> DEKRLHFGNGHLKLPGLRTYVDPHTYEDPTQTVHEFAKELDATNISIDKVVGAGEFGEV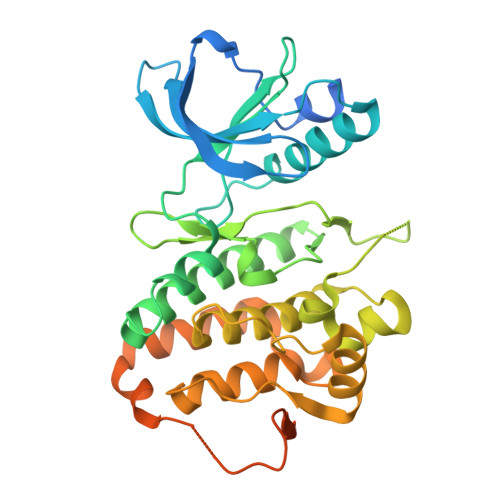CSGRLKLPSKKEISVAIKTLKVGYTEKQRRDFLGEASIMGQFDHPNIIRLEGVVTKSKPVMIVTEYMENGSLDSFLRKHDAQFTVIQLVGMLRGIASGMKYLSDMGYVHRDLAARNILINSNLVCKVSDFGLSRVLEDDPEAAYTTRGGKIPIRWTSPEAIAYRKFTSASDVWSYGIVLWEVMSYGERPYWEMSNQDVIKAVDEGYRLPPPMDCPAALYQLMLDCWQKDRNNRPKFEQIVSILDKLIRNPGSLKIITSAAARPSNLLLDQSNVDITTFRTTGDWLNGVWTAHCKEIFTGVEYSSCDTIAKIS5'-O-{[5-(7-hydroxy-3-oxo-3H-phenoxazin-2-yl)pentanoyl]sulfamoyl}adenosine | C27 H27 N7 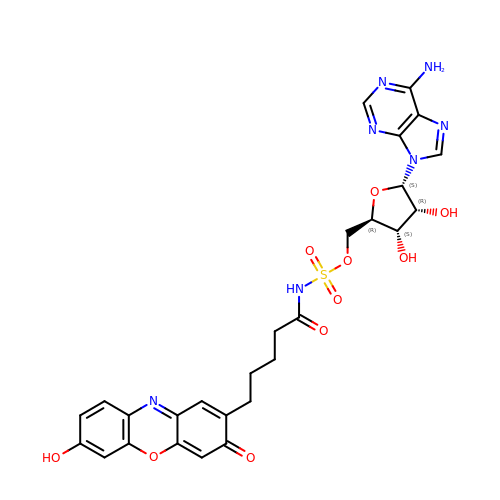O10 S | INHRVYHMUNZSSB-PKDYZCKRSA-N>MRGSHHHHHHGSLSSSPSEILQELGKGSTHPQPGVSPPAAPAAPGPKDGPGETDAFGNSEGKELVASGENKIKQGLLPSLEDLLFYTIAEGQEKIPVHKFITALKSTGLRTSDPRLKECMDMLRLTLQTTSDGVMLDKDLFKKCVQSNIVLLTQAFRRKFVIPDFMSFTSHIDE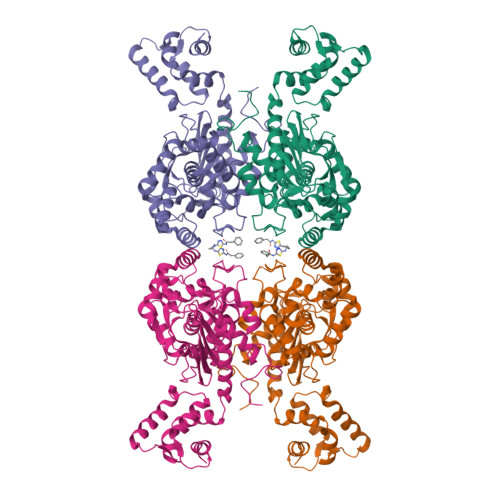LYESAKKQSGGKVADYIPQLAKFSPDLWGVSVCTVDGQRHSTGDTKVPFCLQSCVKPLKYAIAVNDLGTEYVHRYVGKEPSGLRFNKLFLNEDDKPHNPMVNAGAIVVTSLIKQGVNNAEKFDYVMQFLNKMAGNEYVGFSNATFQSERESGDRNFAIGYYLKEKKCFPEGTDMVGILDFYFQLCSIEVTCESASVMAATLANGGFCPITGERVLSPEAVRNTLSLMHSCGMYDFSGQFAFHVGLPAKSGVAGGILLVVPNVMGMMCWSPPLDKMGNSVKGIHFCHDLVSLCNFHNYDNLRHFAKKLDPRREGGDQRHSFGPLDYESLQQELALKETVWKKVSPESNEDISTTVVYRMESLGEKS[4x]> APARGTLLTSNFLTSYTRDAISAMLASGSQPASGSQPEQAKCNVRVAEFTYATIGVEGEPATASGVLLIPGGERCSGPYPLLGWGHPTEALRAQEQAKEIRDAKGDDPLVTRLASQGYVVVGSDYLGLGKSNYAYHPYLHSASEASATIDAMRAARSVLQHLKTPLSGKVMLSGYSQGGHTAMATQREIEAHLSKEFHLVA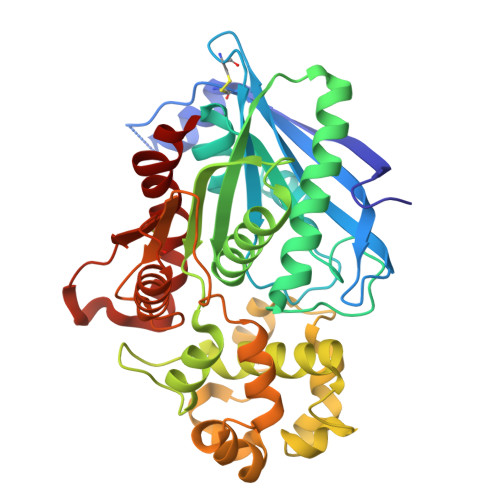SAPISGPYALEQTFLDSWSGSNAVGENTFGILLGSYAIVAMQHTYKNIYLEPGQVFQDPWAAKVEPLFPGKQSLTDMFLNDTLPSIDKVKSYFQPGFYSDFPSNPANPFRQDLARNNLLEWAPQTPTLLCGSSNDATVPLKNAQTAIASFQQRGSNQVALVDTGTGNASDNSAFAHMLTKESCIVVVRDQLLDKQR>[2x]MGIQGLAKLIADVAPSAIRENDIKSYFGRKVAIDA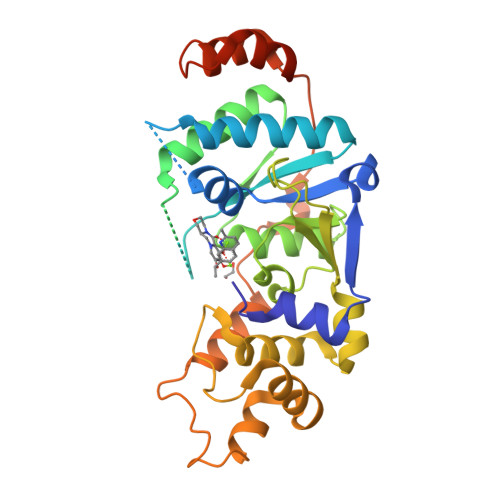SMSIYQFLIAVRQGGDVLQNEEGETTSHLMGMFYRTIRMMENGIKPVYVFDGKPPQLKSGELAKRSERRAEAEKQLQQAQAAGAEQEVEKFTKRLVKVTKQHNDECKHLLSLMGIPYLDAPSEAEASCAALVKAGKVYAAATEDMDCLTFGSPVLMRHLTASEAKKLPIQEFHLSRILQELGLNQEQFVDLCILLGSDYCESIRGIGPKRAVDLIQKHKSIEEIVRRLDPNKYPVPENWLHKEAHQLFLEPEVLDPESVELKWSEPNEEELIKFMCGEKQFSEERIRSGVKRLSKSRQGSTLEVLFQ> TVAAYNLTWKSTNFKTILEWEPKPVNQVYTVQISTKSGDWKSKCFYTTDTECDLTDEIVKDVKQTY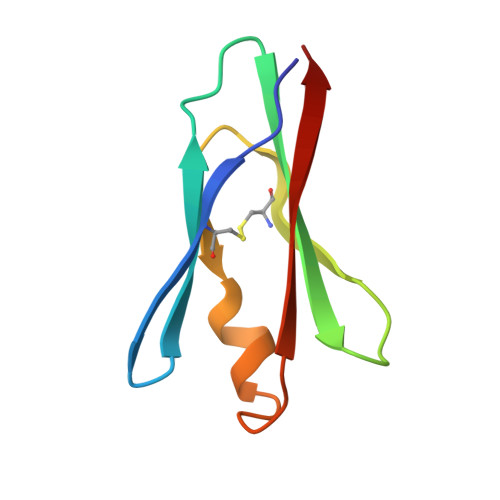LARVFSYPA>[2x]AQFLHTQVGRGLLGAVVNPLGEVTDKFAVTDNSEILYRPVDNAPPLYSERAAIEKPFLTGIKVIDSLLTCGEGQRMGIFASAGCGKTFLMNMLIEHSGADIYVIGLIGERGEEVTETVDYLKNSEKKSRCVLVYATSDYSSVDRCNAAYIATAIAEFFRTEGHKVALFIDSLTRYARALRDVALAAGESPARRGYPVSVFD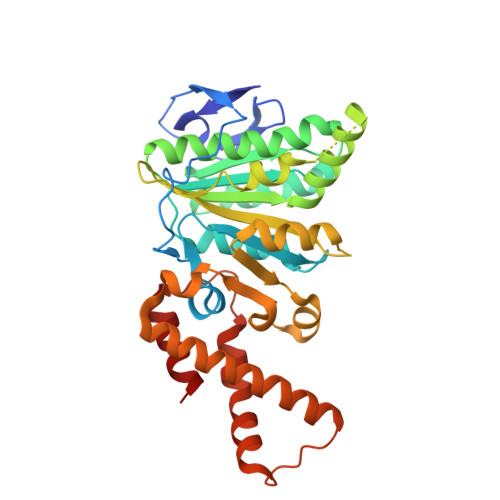SLPRLLERPGKLKAGGSITAFYTVLLEDDDFADPLAEEVRSILDGHIYLSRNLAQKGQFPAIDSLKSISRVFTQVVDEKHRIMAAAFRELLSEIEELRTIIDFGEYKPGENASQDKIYNKISVVESFLKQDYRLGFTYEQTMELIGETIR8-{[2-(1,1-dioxo-1lambda~6~,4-thiazinan-4-yl)ethyl]sulfanyl}-1,3-dimethyl-3,7-dihydro-1H-purine-2,6-dione | C13 H19 N5 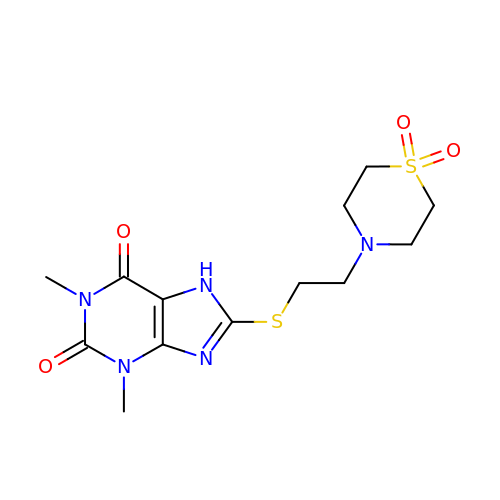O4 S2 | YPZHYYKYMSTZFD-UHFFFAOYSA-N>MPTNQDLQLAAHLRSQVTTLTRRLRREAQADPVQFSQLVVLGAID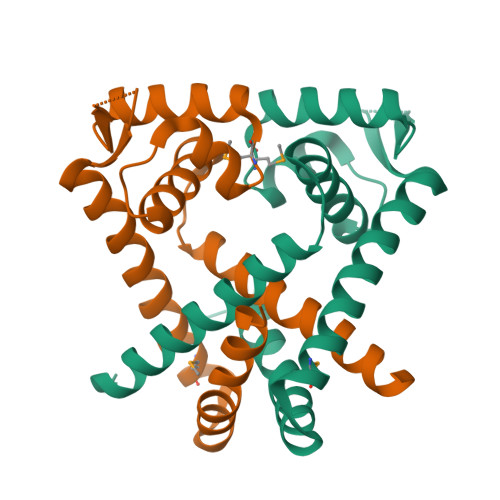RLGGDVTPSELAAAERMRSSNLAALLRELERGGLIVRHADPQDGRRTRVSLSSEGRRNLYGNRAKREEWLVRAMHACLDESERALLAAAGPLLTRLAQFEEP[4x]>MQPPPPGPLGDCLRDWEDLQQDFQNIQETHRLYRLKLEE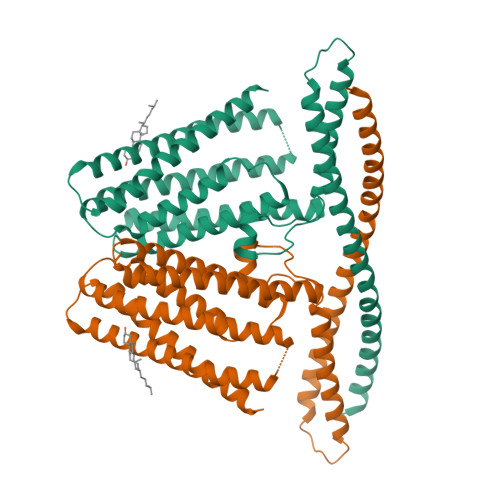LTKLQNNCTSSITRQKKRLQELALALKKCKPSLPAEAEGAAQELENQMKERQGLFFDMEAYLPKKNGLYLSLVLGNVNVTLLSKQAKFAYKDEYEKFKLYLTIILILISFTCRFLLNSRVTDAAFNFLLVWYYCTLTIRESILINNGSRIKGWWVFHHYVSTFLSGVMLTWPDGLMYQKFRNQFLSFSMYQSFVQFLQYYYQSGCLYRLRALGERHTMDLTVEGFQSWMWRGLTFLLPFLFFGHFWQLFNALTLFNLAQDPQCKEWQVLMCGFPFLLLFLGNFFTTLRVVHHKFHSQRHGSKKD[2x]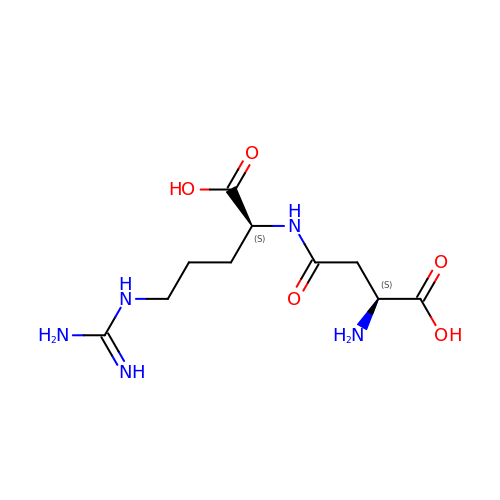(2~{S})-4-[[(2~{S})-5-[[azanyl($l^{4}-azanylidene)methyl]amino]-1-$l^{1}-oxidanyl-1-oxidanylidene-pentan-2-yl]amino]-2-$l^{2}-azanyl-4-oxidanylidene-butanoic acid | C10 H19 N5 O5 | QCGCETFHYOEVAI-WDSKDSINSA-N>[4x]MDIIIK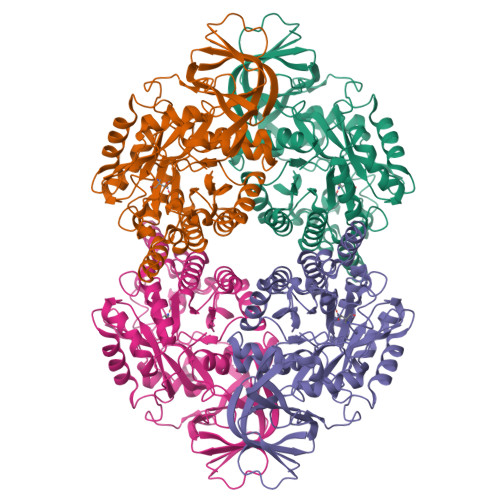NGTIVTADGISRADLGIKDGKITQIGGALGPAERTIDAAGRYVFPGGIDVHTHVETVSFNTQSADTFATATVAAACGGTTTIVDFCQQDRGHSLAEAVAKWDGMAGGKSAIDYGYHIIVLDPTDSVIEELEVLPDLGITSFKVFMAYRGMNMIDDVTLLKTLDKAVKTGSLVMVHAENGDAADYLRDKFVAEGKTAPIYHALSRPPRVEAEATARALALAEIVNAPIYIVHVTCEESLEEVMRAKSRGVRALAETCTHYLYLTKEDLERPDFEGAKYVFTPPARAKKDHDVLWNALRNGVFETVSSDHCSWLFKGHKDRGRNDFRAIPNGAPGVEERLMMVYQGVNEGRISLTQFVELVATRPAKVFGMFPQKGTIAVGSDADIVLWDPEAEMVIEQTAMHNAMDYSSYEGHKVKGVPKTVLLRGKVIVDEGSYVGEPTDGKFLKRRKYKQ>[2x]MKPLYRQLKSSHYSSDYSSPGYLAAEAVYAEIGYELDTLLKQNPGYANTAAVRMSLALLKTGISFKGRLPIKKGAYKGKTIEP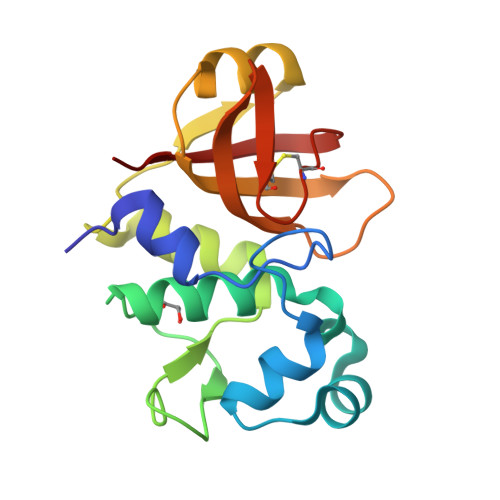GAKLLADQLHRSSSFGKAKIFFNAPDAEKGIGNKKGVVFFNKITNYDGGHIDLIEPENSLLTCHSHCYFNCKEVWFWELS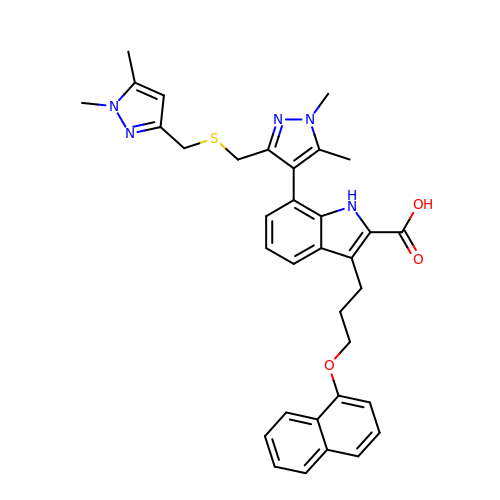7-[3-[(1,5-dimethylpyrazol-3-yl)methylsulfanylmethyl]-1,5-dimethyl-pyrazol-4-yl]-3-(3-naphthalen-1-yloxypropyl)-1~{H}-indole-2-carboxylic acid | C34 H35 N5 O3 S | GMZVNHFKWDLAJN-UHFFFAOYSA-N> GAMVETKCPNLDIVTSSGEFHCSGCVEHMPEFSYMYWLAKDMKSDEDTKFIEHLGDGINEDETVRTTDGGITTLRKVLHVTDTNKFAHYRFTCVLTTLDGVSKKNIWLK;> GYFGKLESKLSVIRNLNDQVLFIDQGNRPLFEDMTDSDSRDNAPRTIFIISMYKDSQPRGMAVTISVKSEKISTLSSENKIISFKEMNPPDNIKDTKSDIIFFQRSVPGHDNKMQFESSSYEGYFLASEKERDLFKLILKKEDELGD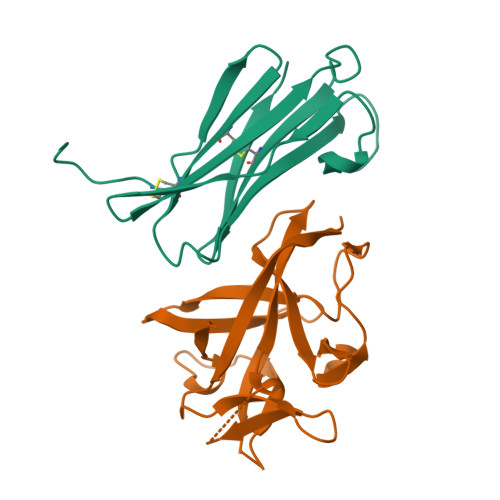RSIMFTVQNED2-{[(1R)-1-(6-nitro-2H-1,3-benzodioxol-5-yl)ethyl]sulfanyl}ethyl 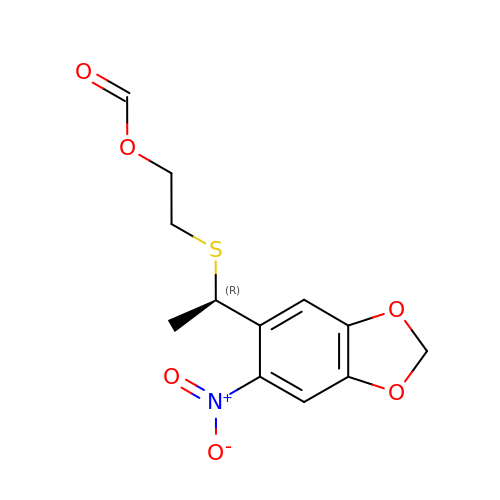formate | C12 H13 N O6 S | OAPSBASJSSKBSD-MRVPVSSYSA-N> MGAQVSSQKVGAHENTNVATGGSTVNYTTINYYKD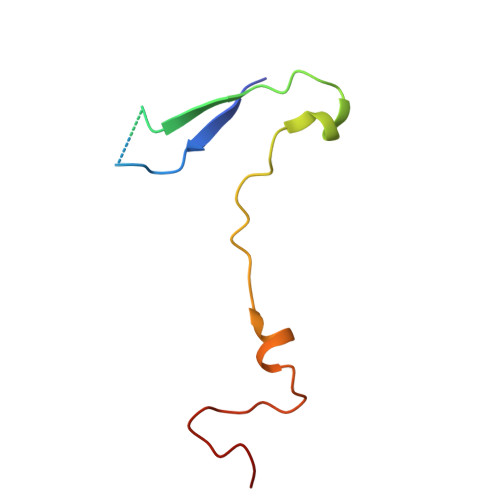SASNAASKLDFSQDPSKFTEPVKDIMIKTAPALN> MVGGGGVKFIEMDIRDKEAYELAKEWFDEVVVSIKFN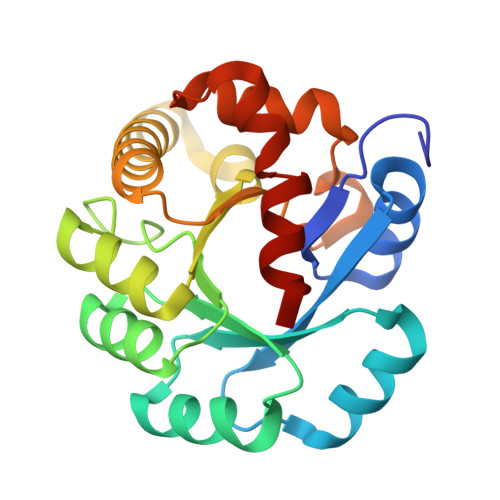EEVDKEKLREARKEYGKVAILLSNPKPSLVRDTVQKFKSYLIYVESNDLRVIRYSIEKGVDAIISPWVNRKDPGIDHVLAKLMVKKNVALGFSLRPLLYSNPYERANLLRFMMKAWKLVEKYKVRRFLTSSAQEKWDVRYPRDLISLGVVIGMEIPQAKASISMYPEIILKRLKY(1S)-1,5-anhydro-1-(5-phenyl-1H-imidazol-2-yl)-D-glucitol 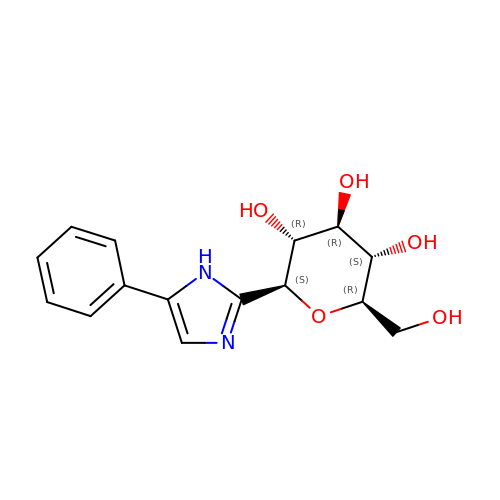| C15 H18 N2 O5 | QJGQTBOHSOZKLJ-RKQHYHRCSA-N> MTQSLFQPITLGALTLKNRIVMPPMTRSRASQPGDVANHMMAIYYAQRASAGLIVSEGTQISPTAKGYAWTPGIYTPEQIAGWRIVTEAVHAKGCAIFAQLWHVGRVTHPDNIDGQQPISSSTLKAENVKVFVDNGSDEPGFVDVAVPRAMTKADIAQVIADYRQAALNAMEAGFDGIELHAANGYLINQFIDSEANNRSDEYGGSLENRLRFLDEVVAALVDAIGAERVGVRLAPLTTLNGTVDADPILTYTAAAALLNKHR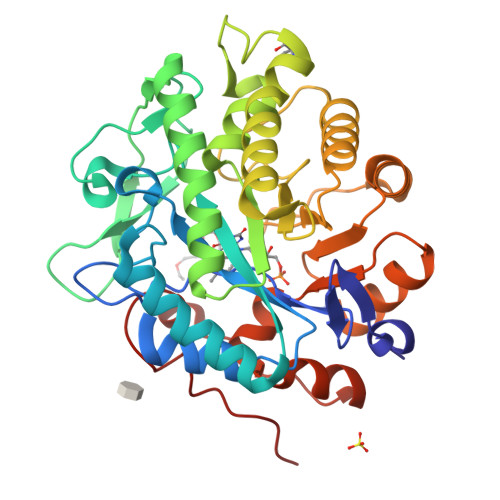IVYLHIAEVDWDDAPDTPVSFKRALREAYQGVLIYAGRYNAEKAEQAINDGLADMIGFGRPFIANPDLPERLRHGYPLAEHVPATLFGGGEKGLTDYPTYQA Inteins are dynamic intervening protein elements that invade at the DNA level and are transcribed and translated along with the host protein. DnaB is the replicative helicase in bacteria and an essential component of the replication machinery. The two inteins in the dnaB gene of M. smegmatis (Msm) are different from each other in sequence, insertion site, and splicing mechanism. The first Msm intein, DnaBi1, lacks a HEN, necessary for invasion of novel sites, and is considered a mini-intein.

To understand the mechanism of disulfide bond formation, a crystal structure of the class 3 DnaBi1 intein was solved to 1.95 Å resolution. Class 3 inteins have several unique attributes, most notably three highly conserved residues in splicing blocks B, F, and G, termed the WCT triplet, that characterizes this class. This structure displayed the classic intein shape, with the β-strand fold indicative of the Hedgehog/Intein (HINT) domain. Class 3 inteins lack a nucleophilic residue at the start of the intein sequence, instead using a conserved internal block F cysteine (top). This internal cysteine (Cys118 for DnaBi1) attacks the N-extein–intein junction (step 1), akin to Cys1 of class 1 inteins. The catalytic center of DnaBi1 is composed of several key residues, including the WCT triplet (left). Catalytic Cys118 is centrally positioned in the active site (left), allowing interactions with both splice junctions. One of the three DnaBi1 molecules within the asymmetric unit, chain B, showed the thiol sidechain of Cys118 adopting two distinct conformations, a and b. Conformation a of Cys118 has 36% occupancy and is the unique orientation for this structure, while conformation b has 64% occupancy and is representative of the Cys118 orientation in the two other molecules in the asymmetric unit. However, both Cys118 conformations are distant from Cys48 (Cys118a, 11.0 Å and Cys118b, 12.1 Å). The thiol sidechains for both residues also rotate inward towards each other. This modeling suggests that subtle conformational shifts can bring the cysteines within proximity and implies that the β-strand containing Cys48 is likely responsible for closing that distance.

>[3x]ALALDTPLPTPSGWTTMGDVAVGDHLLGPDGEPTRVVADTDVMLGRPCYVVEFSDGTAIVADAQHQWPTEHGVRITANLRAGMHTVVSASGGRGGTALLAPAVQITAVRRRPSVPVRCVEVDNPEHLYLAGPGMVPTHN> MTGFTPDAPVLHEIKNHSEELTKAEAGVAAFAAKRNNRWYPKFHIASNGGWINDPNGLCFYKGRWHVFYQLHPYGTQWGPMHWGHVSSADMVNWKREPIMFAPSLEEEKDGVFSGSAVIGDDGKLKFYYTGHRWANGKDNTGGDWQVQMLAEPDNDELTSATKRGMVIDCPTDKVNHHYRDPKVWKTGDKWYMTFGVSSAEKRGQMWLFSSDDMVKWTYEQVLFEHPDSNVFMLECPDFFPIKDVEGNEKWVIGFSAMGAKPSGFMNRNVNNAGYMIGTWTPGEQFKPETEFRLWDCGHNYYAPQSFNDGKRQIVYGWMSPFVEPIPMQDDGWCGNLTLPREITLGADGDLHTAPVAEMEGLREDTVDFGAIDLDVSGEKTIVDDAEAVEIEMTIDLANSTAERAGLRVHATEDGAYTSVAYDDQIGRVVVDRQANAQGDRGYRTAPLSEAELAAGELKLRVYVDRGCVEVYVNDGRQVLSSYSYASEGPRAI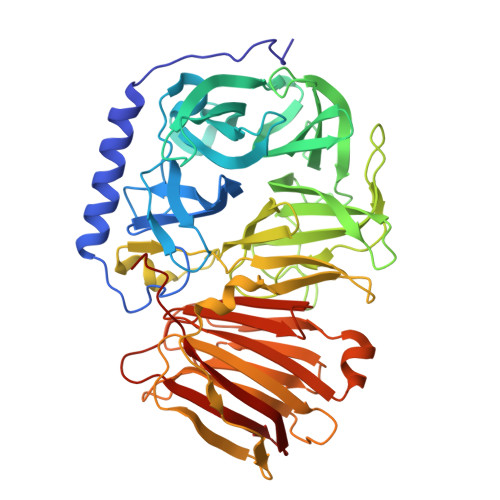KLVAESGTLKVKSLVLHHMKSIGLE4-(3-methylpyridin-4-yl)-6-(trifluoromethyl)-1H-indazole 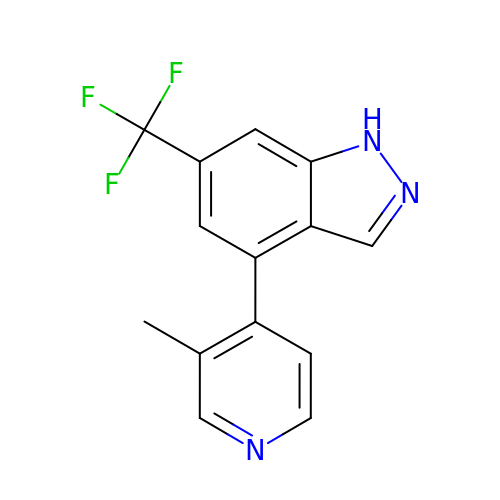| C14 H10 F3 N3 | SERKGWYXQDCJCM-UHFFFAOYSA-N> MKKMMLSVAAVATLMAFAAPVATAKEATWVTDKPLTLKIHMHFRDKWVWDENWPVAKESFRLTNVKLQSVANKAATNSQEQFNLMMASGDLPDVVGGDNLKDKFIQYGQEGAFVPLNKLIDQYAPHIKAFFKSHPEVERAIKAPDGNIYFIPYVPDGVVARGYFIREDWLKKLNLKPPQNIDELYTVLKAFKEKDPNGNGKADEVPFIDRHPDEVFRLVNFWGARSSGSDNYMDFYIDNGRVKHPWAE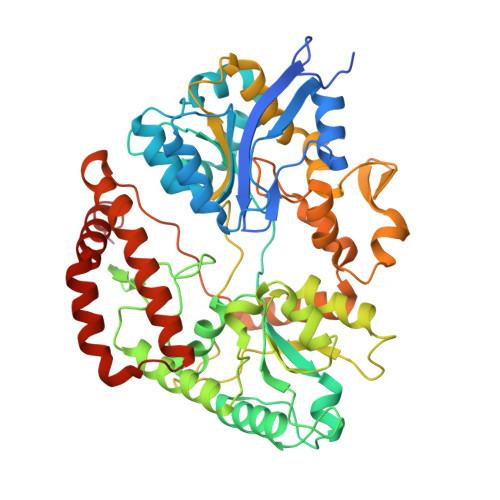TAFRDGMKHVAQWYKEGLIDKEIFTRKARAREQMFGGNLGGFTHDWFASTMTFNEGLAKTVPGFKLIPIAPPTNSKGQRWEEDSRQKVRPDGWAITVKNKNPVETIKFFDFYFSRPGRDISNFGVPGVTYDIKNGKAVFKDSVLKSPQPVNNQLYDMGAQIPIGFWQDYDYERQWTTPEAQAGIDMYVKGKYVMPGFEGVNMTREERAIYDKYWADVRTYMYEMGQAWVMGTKDVDKTWDEYQRQLKLRGLYQVLQMMQQAYDRQYKN>MAAEEGAVIACHTKQEFDTHMANGKDTGKLVIIDFTASWCGPCRVIAPVFAEYAKKFPGAIFLKVDVDELKDVAEAYNVEAMPTFLFIKDGEKVDSVVGGRKDDIH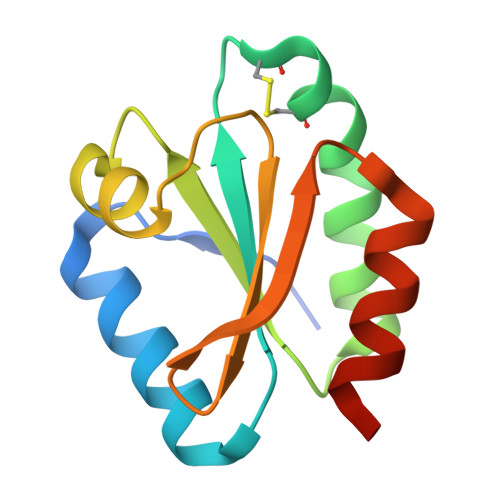TKIVALMGSAST[4x]(1R)-1-benzyl-1-methyl-1-(2-{[4-(1-methylethyl)phenyl]amino}-2-oxoethyl)-2-{(2S)-4-methyl-2-[(trifluoroacetyl)amino]pentanoyl}diazanium 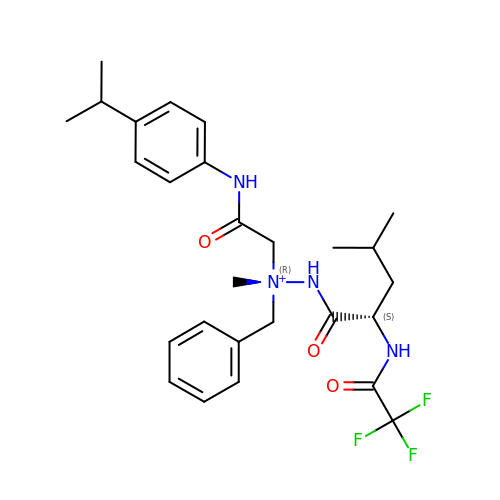| C27 H36 F3 N4 O3 | HTEHUHSQPIQBEG-OHWKKVTOSA-O>MQTPLSLRERDARVIAEIGRLRFSPLSLIGGKGNRLIEEGGRSILDLSGSAGPAALGYGHPAIVEAVEKSVRDMAGASLLLYPNEAAVSLAEDLLRITPGNGERRVWFGHSGSDANDCAVRVLTAATKRSRIISFIGSYHGNLTGSMGISGHTAMTHTLPRPGVLLLPYPDPFRPRFSAEAVLELLDYHFATSCPPEQVAAVFIEPILSDGGLVVPPPAFLEALQDRCRKHGILVVVDEVKVGLGRTGLMHCFQHEGLEPDMVVFGKGLGGGLPLSAVVGPQWVMDHAPAFVLQTTAGNPVATAAGRAVLNTIERQGLAQRSERVGGIFADRLRRL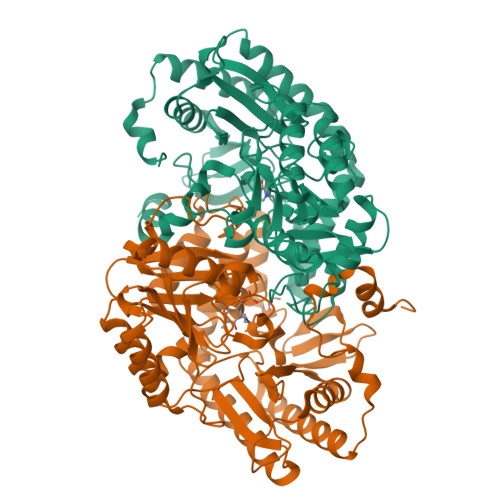SDKHSIIGDVRGRGLAIGVDLVSDRGSREPAPVTTTAKIIYRGYQLGAAFTYVGLNANVLEFMPPLTLTEPEIDEAADIVDQAIGDVLDGKVADSDVAHFMMW[4x]>[2x]MTPSRPSPDFPDGGFVQVRGARQHNLKDISVKVP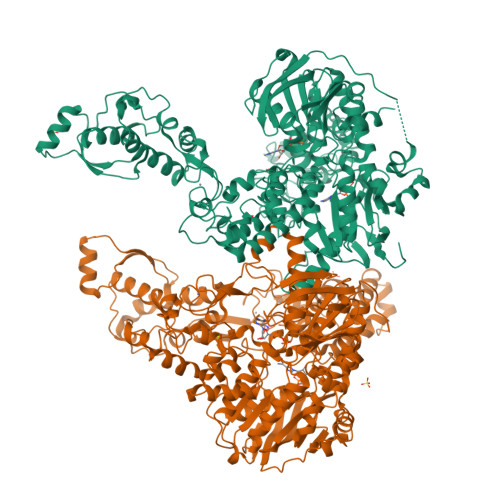RDALVVFTGVSGSGKSSLAFGTLYAEAQRRYLESVSPYARRLFNQAGVPDVDAIDGLPPAVALQQARGTPTARSSVGSVTTLSNLLRMLYSRAGDYPPGQGIVYAEGFSPNTPEGACPECHGLGRVYTVTEDSMVPDPSLTIRERAVAAWPQAWGGQNQRDILVTLGIDVDVPWRELPEETRHWILFTDEQPVVPVYPGLTPAETQRALKKKMEPSYMGTFSSARRHVLHTFANTESASMKKRVQGYMISEECPLCHGKRLRQEALNVTFAGLDITELSRLPLARVSELLRPYAEEREPGHAERVKNRPEQAIALQRMAADLVKRLDVLLHLGLGYLGLDRSTPTLSPGELQRLRLATQLYSNLFGVVYVLDEPSAGLHPADTEALLSALENLKRGGNSLFVVEHDLDVIRRADWLVDVGPEAGEKGGEILYSGPPEGLKHVPESQTGQYLFADRHTEPHTPREPAGWLELNGVTRNNLDNLDVRFPLGVMTSVTGVSGSGKSTLVSQALVDALAAHFGQPVNPDPEDDEDPADHTAGSARLGGDLAQITRLVRVDQKPIGRTPRSNMATYTGLFDQVRKLFAATPLAKKRGYNAGRFSFNVKGGRCEHCQGEGWVMVELLFLPSVYAPCPVCHGTRYNAETLEVEYRGKNIADVLALTVDEAHDFFADESAIFRALDTLREVGLGYLRLGQPATELSGGEAQRIKLATELRRSGRGGTVYVLDEPTTGLHPADVERLQRQLVKLVDAGNTVIAVEHKMQVVAASDWVLDIGPGAGEDGGRLVAQGTPAEVAQAAGSVTAPYLRAALR> MGPYRRLWF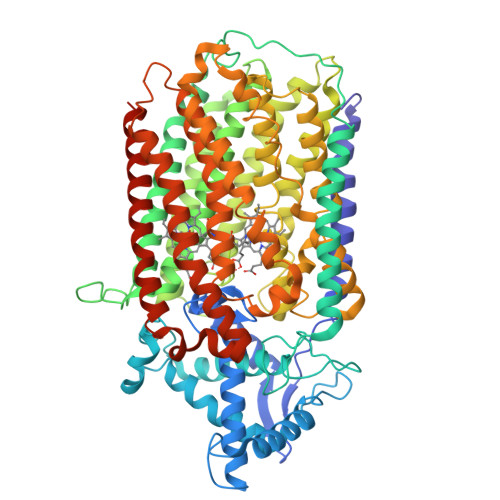TLIAVLAVTFALLGFYGGEVYRQAPPIPEEVASADGTRLFGRDDILDGQTAWQSIGGMQLGSIWGHGAYQAPDWTADWLHRELMAWLDLAARDAHGRDYGQLDAPAQAALREQLKAEYRANRADAAGGKLTLSPRRAQAVAQTEAYYDQLFSDAPALHRSRENYAMKENTLPDANRRRQMTHFFFWTAWAAGTEREGTSVTYTNNWPHEPLIGNHPSSENVMWSIISVVVLLAGIGLLIWAWAFLRGKEEDEPPAPARDPLTTFALTPSQRALGKYLFLVVALFGFQVLLGGFTAHYTVEGQKFYGIDLSQWFPYSLVRTWHIQSALFWIATGFLAAGLFLAPLINGGRDPKYQKAGVDILFWALVLVVVGSFAGNYLAIAQIMPPDLNFWLGHQGYEYVDLGRLWQIGKFAGICFWLVLMLRGIVPALRTPGGDKNLLALLTASVGAIGLFYGAGFFYGERTHLTVMEYWRWWIVHLWVEGFFAVFATTALAFIFSTLGLVSRRMATTASLASASLFMLGGIPGTFHHLYFAGTTTPVMAVGASFSALEVVPLIVLGHEAWENWRLKTRAPWMENLKWPLMCFVAVAFWNMLGAGVFGFMINPPVSLYYIQGLNTTPVHAHAALFGVYGFLALGFTLLVLRYIRPQYALSPGLMKLAFWGLNLGLALMIFTSLLPIGLIQFHASVSEGMWYARSEAFMQQDILKTLRWGRTFGDVVFLLGALAMVVQVILGLLSGKPAAAEPVLRAEPARRL> MHHHHHHLVPRGSVSKRDKRISLDDAVGELRSGMTIGIGGWGSRRKPMALVRALLRSDVTDLTVVTYGGPDLGLLCSAGKVTKAYYGFVSLDSAPFYDPWFAKARTAGEIAVREMDAGMVKCGLEAAAARLPFLPIRAGLGSDVRRFWGDELRTVTSPYPDASGKSETLIAMPALNLDAALVHLNLGDKHGNAAYTGVDPYFDDLYCAAAEKRFVSVERVVETEELVKTVPLQNLILNRMMVDGVVEAPNGAHFTLAGDSYGRDEKFQRHYAESAKTPQAWQQFVATYLSGSEDDYQAAVKKFAEEQA;> MSETITEVTRAEYCAIACADIFSGAGEIMASPMATLPLIGARLARLTTEPDLLITDGEALIFADTPAVGAKAPIEGWMPFRKVFDVVASGRRHVVMGANQIDRHGNQNLSAFGPLQQPTRQMFGVRGAPGNTINHPTSYWVGKHTSRVFCDT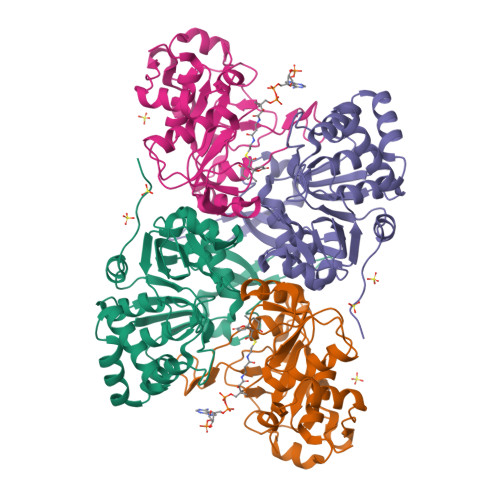VDIVSGVGYDQIDPENPAYRFHHLHRVVSNLGVFDFGGPDHTFRALSLHPGVTADQVADNTSFEVAGLADAGVTREPTDEELRLIREVLDPRSLRDREVSV>IVHREHHESREEVSVSSGKNNPFYFNSDRWFRTLYRNEWGHIRVLQRFDQRSKQMQNLENYRVVEFKSKPNTLLLPHHADADFLLVVLNGTAVLTLVNPDSRDSYILEQGHAQKIPAGTTFFLVNPDDNENLRIIKLAIPVNNPHRFQDFFLSSTEAQQSYLRGFSKNILEASFDSDFKEINRVLFGEERQQQQGEESREEGVIVELKREQIQELMKHAKSSSRKELSSQDEPFNLRNSKPIYSNKFGRWYEMTPEKNPQLKDLDVFISSVDMKEGALLLPHYSSKAIVIMVINEGEAKIE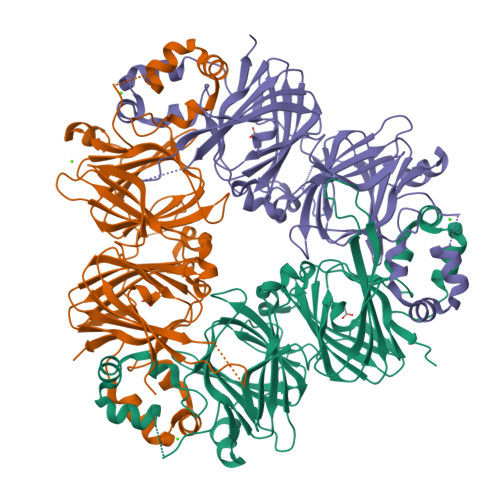LVGLSDQQQQKQQEESLEVQRYRAELSEDDVFVIPAAYPVAINATSNLNFFAFGINAENNRRNFLAGGKDNVMSEIPTEVLEVSFPASGKKVEKLIKKQSESHFVDAQPEQQQREEGHKGRKGSLSSILGSLY[3x]>[2x]MNLLRRSGKRRRSESGSDSFSGSGGDSSASPQFLSGSVLSPPPGLGRCLKAAAAGECKPTVPDYERDKLLLANWGLPKAVLEKYHSFGVKKMFEWQAECLLLGQVLEGKNLVYSAPTSAGKTLVAELLILKRVLEMRKKALFILPFVSVAKEKKYYLQSLFQEVGIKVDGYMGSTSPSRHFSSLDIAVCTIERAN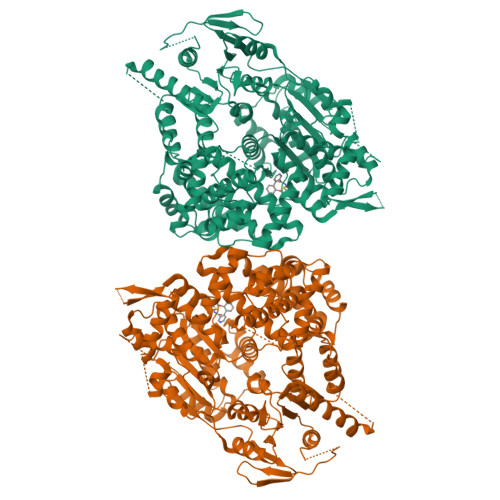GLINRLIEENKMDLLGMVVVDELHMLGDSHRGYLLELLLTKICYITRKSASCQADLASSLSNAVQIVGMSATLPNLELVASWLNAELYHTDFRPVPLLESVKVGNSIYDSSMKLVREFEPMLQVKGDEDHVVSLCYETICDNHSVLLFCPSKKWCEKLADIIAREFYNLHHQAEGLVKPSECPPVILEQKELLEVMDQLRRLPSGLDSVLQKTVPWGVAFHHAGLTFEERDIIEGAFRQGLIRVLAATSTLSSGVNLPARRVIIRTPIFGGRPLDILTYKQMVGRAGRKGVDTVGESILICKNSEKSKGIALLQGSLKPVRSCLQRREGEEVTGSMIRAILEIIVGGVASTSQDMHTYAACTFLAASMKEGKQGIQRNQESVQLGAIEACVMWLLENEFIQSTEASDGTEGKVYHPTHLGSATLSSSLSPADTLDIFADLQRAMKGFVLENDLHILYLVTPMFEDWTTIDWYRFFCLWEKLPTSMKRVAELVGVEEGFLARCVKGKVVARTERQHRQMAIHKRFFTSLVLLDLISEVPLREINQKYGCNRGQIQSLQQSAAVYAGMITVFSNRLGWHNMELLLSQFQKRLTFGIQRELCDLVRVSLLNAQRARVLYASGFHTVADLARANIVEVEVILKNAVPFKSARKAVDEEEEAVEERRNMRTIWVTGRKGLTEREAAALIVEEARMILQQDLVEM Among these, group 21 allergens including Blo t 217, Der p 218 and Der f 219 identified in B. tropicalis, D. pteronyssinus and D. farinae, respectively, are known as mid-tier allergens in the allergic response. The structure of rDer f 21 adopts a bundle of three anti-parallel α-helices similar to the group 21 HDM allergen Blo t 2116, and group 5 HDM allergens including Blo t 514,15 and Der p 512. The crystal structure of rDer f 21 revealed an elongated dimer structure with molecules A and B interacting in a head-to-toe orientation. Helices α1 and α2 form an intermolecular anti-parallel dimeric interface while the C-terminal α-helix (α3) is fully exposed to the solvent.

The structure of rDer f 21 bound to a molecule of PEG 400, rDer f 21PEG400, was determined to 1.5 Å resolution from a crystal belonging to C-centered monoclinic space group C2. The structure contains two molecules per asymmetric unit forming a rDer f 21 dimer. Each molecule of rDer f 21PEG400 is approximately 60 × 17 × 14 Å and forms a coiled coil bundle structure composed of three anti-parallel α-helices denoted as α1 (A14 to T47), α2 (K50 to A78), and α3 (M85 to K113). Structural comparison of two molecules A and B representing the asymmetric unit of the rDer f 21PEG400 crystal structure shows a significant structural deviation localised at the α1 helix of molecule B between residues 20-30. The r.m.s.d. between the two molecules is reaching up to 4.3 Å. The dramatic conformational changes at the helix α1 of the molecule B are caused by the binding of a well-ordered PEG 400 molecule (from the crystallization buffer) in the pocket of the rDer f 21PEG400 molecule. Interestingly, the coordinates of other residues surrounding the ligand binding pocket including F23 and Y66 are well conserved. The conformational changes enable binding of the ligand into the dimer interface cavity, an event which may otherwise be prevented by steric clashes. The binding cavity consists mostly of hydrophobic residues including A70 and three aromatic residues F23, F73, and Y66. The PEG 400 molecule in the cavity of the rDer f 21 dimer interface only forms one hydrogen bond to Y66A (residue Y66 of molecule A) and is further coordinated via several hydrogen bonds with water molecules in the cavity. The lack of direct hydrogen bonds between the PEG 400 molecule and the surrounding residues suggests that the cavity would prioritize a hydrophobic ligand.

>GLVPRGSEDKWRNAFDHMLMEEFEEKMDQIEHGLLMLSEQYKELEKTKSKELKEQILRELTIAENYLRGALKFMQQEAKRTDLNMFERYNFETAVSTIEILVKDLAELAKKVKAVKSD[2x]> LTPDQQTLLHFIMDSYNKQRMPQEITNKILKEEFSAEENFLILTEMATNHVQVLVEFTKKLPGFQTLDHEDQIALLKGSAVEAMFLRSAEIFNKKLPSGHSDLLEERIRNSGISDEYITPMFSFYKSIGELKMTQEEYALLTAIVILSPDRQYIKDREAVEKLQEPLLDVLQKLCKIHQPE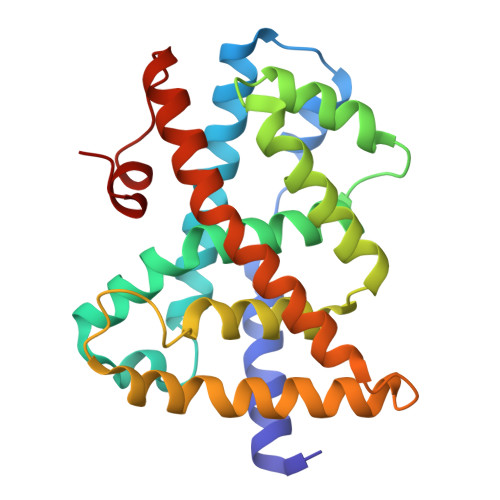NPQHFACLLGRLTELRTFNHHHAEMLMSWRVNDHKFTPLLCEIWDVQ> PGPVPPSTAVRELIEELINITQNQKAPLCNGSMVWSINRTAGMYCA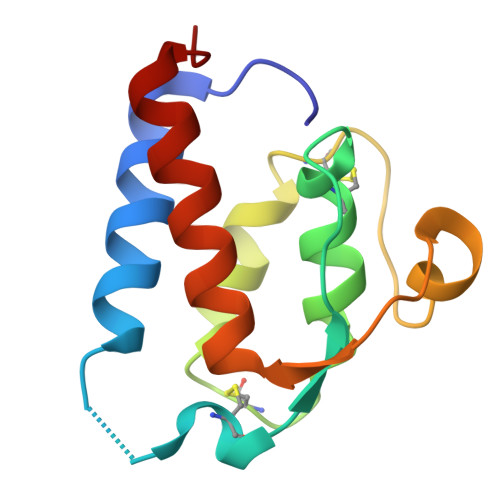ALESLINVSGCSAIEKTQRMLSGFCPHKVSAGQFSSLHVRSSKIEVAQFVKDLLFHLRTLFREGQFN> SDSLSKSPENWMSKLDDGKHLTEINIPGSHDSGSFTLKDPVKSVWAKTQDKDYLTQMKSGVRFFDIRGRASADNMISVHHGMVYLHHELGKFLDDAKYYLSAYPNETIVMSMKKDYDSDSKVTKTFEEIFREYYYNNPQYQNLFYTGSNANPTLKETKGKIVLFNRMGGTYIKSGYGADTSGIQWADNATFETKINNGSLNLKVQDEYKDYYDKKVEAVKNLLAKAKTDSNKDNVYVNFLSVASGGSAFNSTYYYASYINPEIAKTIKANGKARTGWLIVDYAGYT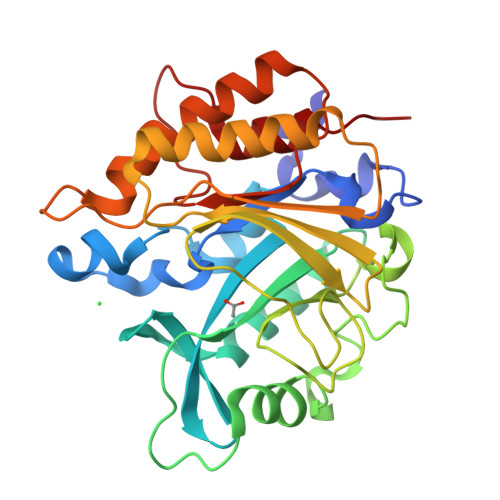WPGYDDIVSEIIDSNKLE>[4x]MRGSHHHHHHGSACQNLNGKVAFVTGGSRGIGAAIVRRLAADGADIAFTYVSASSKNVATALVQELEAKGRRARAIQADSADPAQVRQAVEQAIVQLGPVDVLVNNAGIFLAGPLGEVTLDDYERTMNINVRAPFVAIQAAQASMPDGGRIINIGSCLAERAGRAGVTL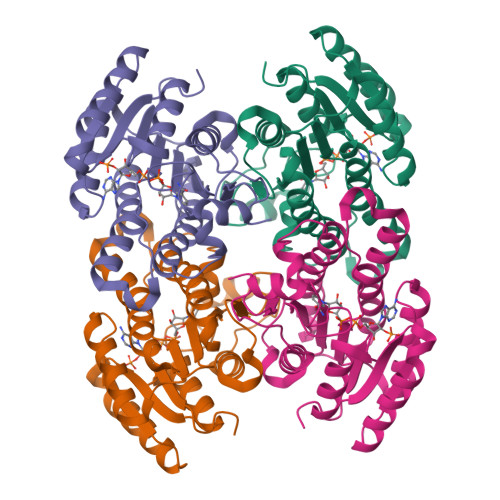YAASKSALLGMTRGLARDLGARGITANVVHPGPIDTDMNPADGERSGELVAVLSLPHYGEVRDIAGMVAFLAGPDGRYVTGASLAVDGGFAA> HHHHHHMPVFHTRTIESILEPVAQQISHLVIMHEEGEVDGKAIPDLTAPVAAVQAAVSNLVRVGKETVQTTEDQILKRDMPPAFIKVENACTKLVQAAQMLQSDPYSVPARDYLIDGSRGILSGTSDLLLTFDEAEVRKIIRVCKGILEYLTVAEVVETMEDLVTYTKNLGPGMTKMAKMIDERQQELTHQEHRVM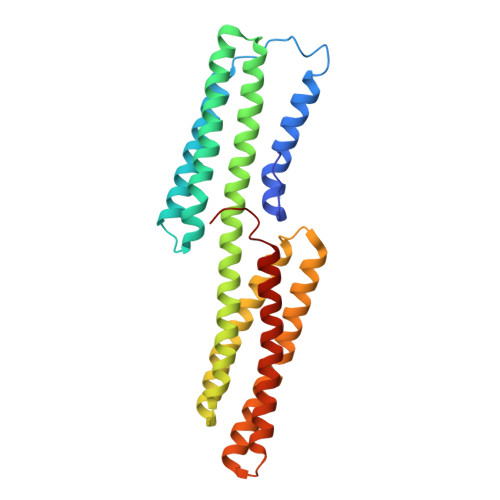LVNSMNTVKELLPVLISAMKIFVTTKNSKNQGIEEALKNRNFTVEKMSAEINEIIRVLQLTSWDEDAW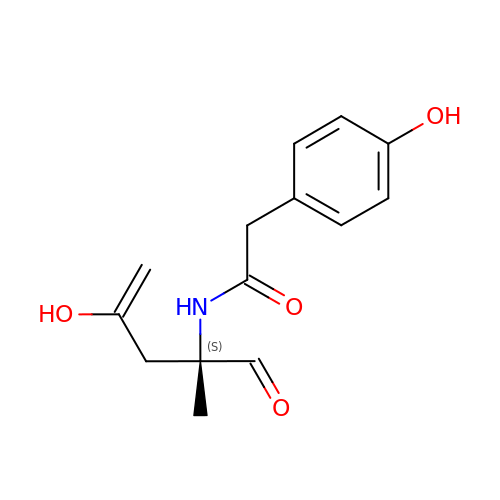2-(4-hydroxyphenyl)-~{N}-[(2~{S})-2-methyl-4-oxidanyl-1-oxidanylidene-pent-4-en-2-yl]ethanamide | C14 H17 N O4 | RSUSHGHDXWZFTH-AWEZNQCLSA-N>MYELYTLLAEYYDTIYRRRIERVKAEIDFVEEIFKEDAKREVRRVLDLACGTGIPTLELAERGYEVVGLDLHEEMLRVARRKAKERNL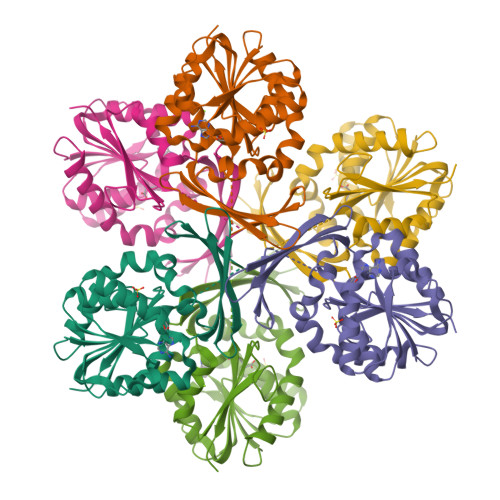KIEFLQGDVLEIAFKNEFDAVTMFFSTIMYFDEEDLRKLFSKVAEALKPGGVFITDFPCWFYGGRDGPVVWNEQKGEEKLVIMDWREVEPAVQKLRFKRLVQILRPNGEVKAFLVDDELNIYTPREVRLLAEKYFEKVKIYGNLKRELSPNDMRYWIVGIAKSF[3x]> TSELRICRIDKESGPCTGGEELYLLCDKVQKEDISVRFSTASWEGRGDFSQADV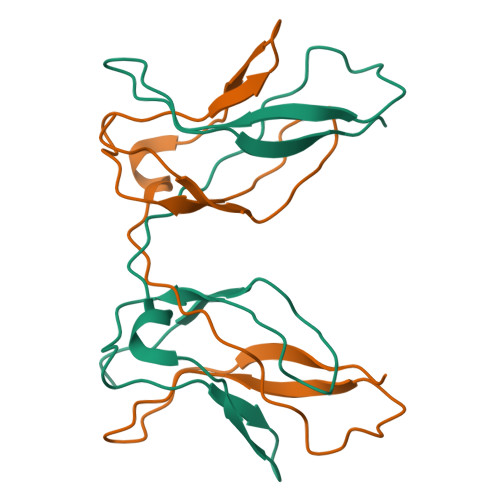HRQFAIVFKTPPYEDLEISEPVTVNVQLQRLTDGECSEPLPFTYLPR>HHHHHHSSGLVPRGSHMENPLQKARILVNQLEKYLDRYAKEYDVEHLAGPQGHLVMHLYKHPDKDMSIKDAEEILHISKSVASNLVKRMEKNGFIAIVPSKTDKRVKYLYLTHLGKQKATQFEIFLEKLHSTMLAG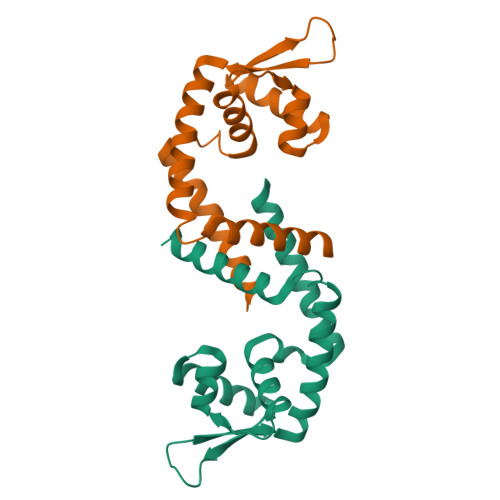ITKEEIRTTKKVIRTLAKNMAMEDFD[4x]>[2x]MKIVIAPDSFKESLTAQQVAEAIKRGFQQSIADVECLLCPVGDGGEGTVDAIRHSLDLEEKCLQVTGSFGQKEVMRYFQKEQLALFEVADLVGLGKIPLEKRNPLQIQTRGIGELIRHLISQEIKEIYIGVGGTASNDGGIGIAAGLGYQFYDEDGNALPACGQSLLNLASVSTENRYKIPEDVHIRILADVVSPLCGHQGAT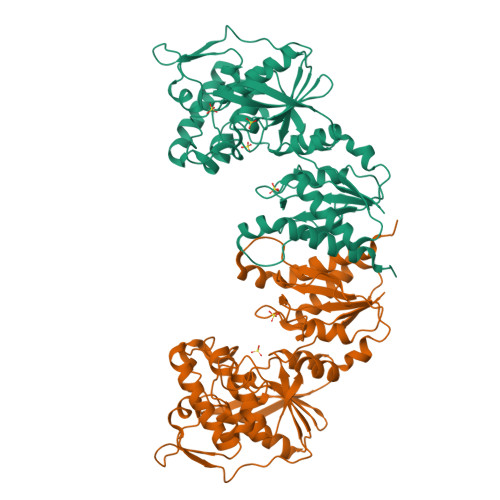YTFGKQKGLDSTMFEVVDQAIQDFYEKVSPATLKLKGAGAGGGIAGGLCAFAQASIVSGIDTCLDLIDFDKKVSDVDLVIVGEGRLDRQSLAGKAPIGVAKRTPVGVPVVAICGSLVEDLPSLPFENIQAAFSILEKSEPLEDSLKNASLYLEHTASNIGHLLNMPKI> MLRNHKLSKVFSATAISLFLSSTAFADTTVRMMHIETDPNVLGVWEEIAKDFEAKNPDIKVNLEFLENEAFKAKLPTLLQSQQKPDLFYSWGGGNFQVRAESGLLEDMEGYSATLNQELSAAGMNAFKIDGKQYGAPYMVSQVGFWYNKKLFKQAGIDGESIQTWDEFLTAIEKLKAAGITPIAVGGADKWPMHFYWSYLAMRAGGQEAFAAAMQDQGDGFAGEAFVRAGEELKRLAALEPFQPGFMAAGYGESAGLFGDYKAAIHLMGDWDYNFQAQQAVDKKGVVDSDLGFMNFPVLKGGAGAGSDTLGGINGFAFAKGAKPEAAKWLEFFLNENSQTKLAEIDQIIPVAKGADKGLKNPFKQKISQTISSAQWHQVFFDQALGADVGGVVNDISVGIVNGDVTPKEAAEQVQEAWEMRLEHHHHHH

The pathway starts with the extracellular decomposition of β-1,3-xylan by two β-1,3-xylanases into β-1,3-xylooligomers, which are mainly internalized by an ATP-binding cassette transporter. The substrate binding protein of this transporter has an L-shaped substrate binding pocket to preferentially bind β-1,3-xylooligomers. XylC comprises two domains (domains I and II) with the substrate bound between the two domains, similar to other SBPs of ABC transporters.

To reveal the mechanism by which XylC preferentially binds β-1,3-XOs, the crystal structures of XylC in complex with β-1,3X2, β-1,3X3, and β-1,4X2, separately, were solved. The three structures are highly similar with root mean square deviations (RMSDs) of 0.18 ~ 0.23 Å. The binding pocket of XylC is L-shaped. In β-1,4-XO-binding proteins, however, the pockets are arc-shaped to accommodate the nearly linear β-1,4-XOs. In the structure of XylC-β-1,4X2, a ~ 45° deviation of xylose 2 was indeed observed compared to that in XylC-β-1,3X3 and XylC-β-1,3X2. The deviation results in the absence or increased distances of hydrogen bonds to Asn68, Trp91, and Asn314, which explains the poor binding affinities of XylC to β-1,4X2. Among all the tested XOs, XylC displayed the highest affinity to β-1,3X4 with a Kd (dissociation constant) value of 1.0 μM, but no binding to β-1,4X4. Its binding affinities to β-1,3X2 and β-1,3X3 were 5.5 times and 29.9 times that of β-1,4X2 and β-1,4X3, respectively, and no binding was detected to xylose.>[3x]ANPLYQKHIISINDLSRDDLNLVLATAAKLKANPQPELLKHKVIASCFFEAST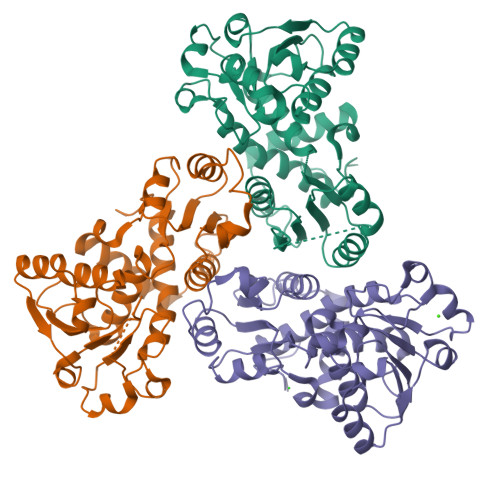RTRLSFETSMHRLGASVVGFSDSANTSLGKKGETLADTISVISTYVDAIVMAHPQEGAARLATEFSGNVPVLNAGDGSNQHPTQTLLDLFTIQETQGRLDNLHVAMVGDLKYGRTVHSLTQALAKFDGNRFYFIAPDALAMPQYILDMLDEKGIAWSLHSSIEEVMAEVDILYMTRVQKERLDPSEYANVKAQFVLRASDLHNAKANMKVLHPLPRVDEIATDVDKTPHAWYFQQAGNGIFARQALLALVLNRDLVL> SVDMALGDLMVSRFSQSSVSLVSNHRYDEDCVSSHDDGDSRRKDSEAKSSSSYGNGTTEGAATATSMAYLPQTIVLCELRHDASEASAPLGTSEIVLVPKWRLKERMKTGCVALVLCLNITVDPPDVIKISPCARIEAWIDPFSMAPPKALETIGKNLSTQYERWQPRARYKVQLDPTVDEVRKLCLTCRKYAKTERVLFHYNGHGVPKPTANGEIWVFNKSYTQYIPLPISELDSW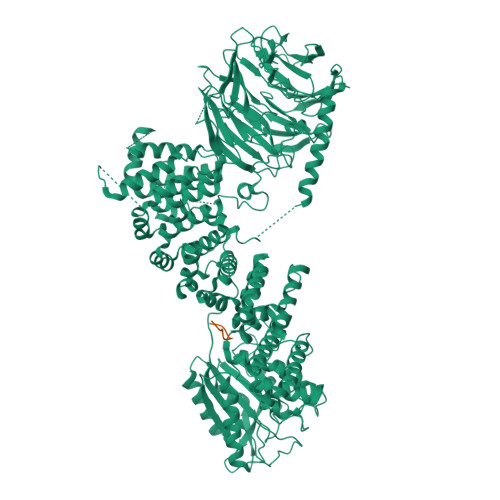LKTPSIYVFDCSAARMILNAFAELHDWGSSGSSGSSRDCILLAACDVHETLPQSVEFPADVFTSCLTTPIKMALKWFCRRSLLKEIIDESLIDRIPGRQNDRKTLLGELNWIFTAVTDTIAWNVLPHELFQRLFRQDLLVASLFRNFLLAERIMRSANCNPISHPMLPPTHQHHMWDAWDMAAEICLSQLPQLVLDPSTEFQPSPFFTEQLTAFEVWLDHGSEHKKPPEQLPIVLQVLLSQCHRFRALVLLGRFLDMGSWAVDLALSVGIFPYVLKLLQTTTNELRQILVFIWTKILALDKSCQIDLVKDGGHTYFIRFLDSSGAFPEQRAMAAFVLAVIVDGHRRGQEACLEANLIGVCLGHLEASRPSDPQPEPLFLQWLCLCLGKLWEDFMEAQIMGREANAFEKLAPLLSEPQPEVRAAAVFALGTLLDIGFDSNKSVVEDEFDDDEKIRAEDAIIKSLLDVVSDGSPLVRAEVAVALARFAFGHKQHLKLAAASYWKPQSSSLLTSLPSIAKFHDPGSATIVSLHMSPLTRASTDSQPVARESRISSSPLGSSGLMQGSPLSDDSSLHSDSGMMHDSVSNGAVHQPRLLDNAVYSQCVRAMFALAKDPSPRIASLGRRVLSIIGIEQVVAKPSKPTGRPGEAADSGLADPLLGASGSERSLLPLSTIYGWSCGHFSKPLLGGADASQEIAAKREEKEKFALEHIAKCQHSSISKLNNNPIANWDTRFETGTKTALLHPFSPIVVAADENERIRVWNYEEATLLNGFDNHDFPDKGISKLCLINELDDSLLLVASCDGSVRIWKNYATKGKQKLVTGFSSIQGHKPGARDLNAVVDWQQQSGYLYASGETSTVTLWDLEKEQLVRSVPSESECGVTALSASQVHGGQLAAGFADGSLRLYDVRSPEPLVCATRPHQKVERVVGLSFQPGLDPAKVVSASQAGDIQFLDLRTTRDTYLTIDAHRGSLTALAVHRHAPIIASGSAKQLIKVFSLQGEQLGIIRYYPSFMAQKIGSVSCLTFHPYQVLLAAGAADSFVSIYTHDNSQAR;> MAGVFDIDLDQPED>[4x]MPERLQVYKCEV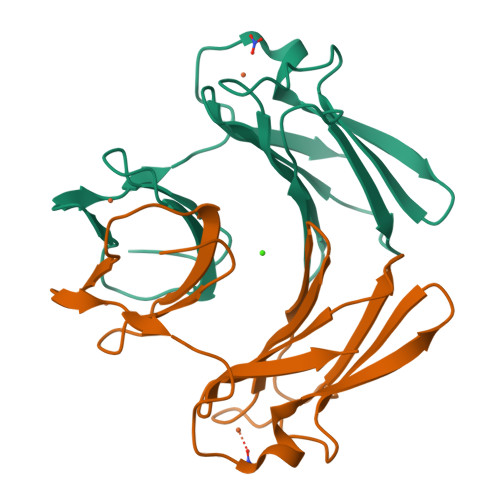CGNIVEVLNGGIGELVCCNQDMKLMSENTVDAAKEKHVPVIEKIDGGYKVKVGAVAHPMEEKHYIQWIELLADDKCYTQFLKPGQAPEAVFLIEAAKVVARAYCNIHGHWKAEN> QDWLTFQKKHITNTRDVDCDNILSTNLFHCKDKNTFIYSRPEPVKAICKGIIASKNVLTTSEFYLSDCNVTSRPCKYKLKKSTNKFCV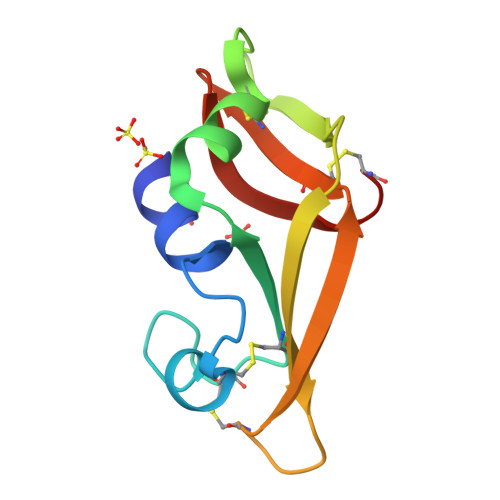TCENQAPVHFVGVGSC2-[3-(2-methoxyphenyl)-3-oxidanylidene-propyl]benzoic 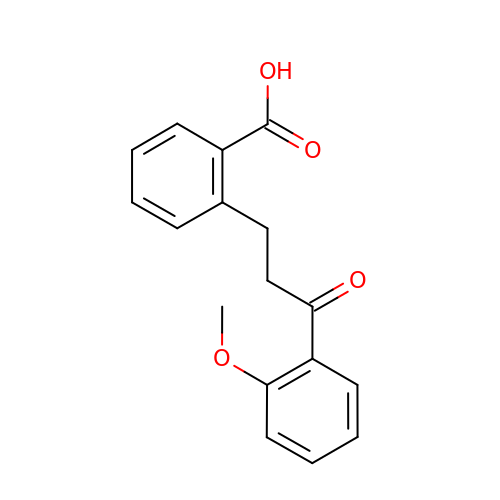acid | C17 H16 O4 | BGYZYPMQNIMFRN-UHFFFAOYSA-N> ME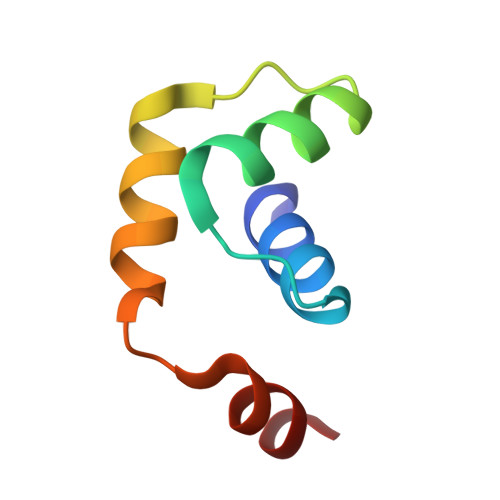YVYAALLLHSVGKEINEENLKAVLQAAGVEPEEARIKALVAALEGVNIDEVIEKAA>GSMAQILPIRFQEHLQLQNLGINPANIGFSTLTMESDKFICIREKVGEQAQVVIIDMNDPSNPIRRPISADSAIMNPASKVIALKAGKTLQIFNIEMKSKMKAHTMTDDVTFWKWISLNTVALVTDNAVYHWSMEGESQPVKMFDRHSSLAGCQIINYRTDAKQKWLLLTGISAQQNRVVGAMQLYSVDRKVSQPIEGHAASFAQFKMEGNAEESTLFCFAVRGQAGGKLHIIEVGTPPTGNQPFPKKAVDVFFPPEAQNDFPVAMQISEKHDVVFLITKYGYIHLYDLETGTCIYMNRISGETIFVTAPHEATAGIIGVNRKGQVLSVCVEEENIIPYITNVLQNPDLALRMAVRNNLAGAEEL[2x];>ETLLDLDFLE[6x]

Clathrin mediates vesicular transport between post‐Golgi membranes in eukaryotes and is targeted to specific membranes by interactions with clathrin adaptor proteins. A total of 3 consensus clathrin‐binding peptide sequences have been identified and structural studies show that each binds distinct sites on the clathrin heavy chain N‐terminal domain (NTD). We have solved high‐resolution structures of NTD bound to peptide motifs from the cellular clathrin adaptors β2 adaptin and amphiphysin plus a putative viral clathrin adaptor, hepatitis D virus large antigen (HDAg‐L). Surprisingly, with each peptide we observe simultaneous peptide binding at multiple sites on NTD and viral peptides binding to the same sites as cellular peptides.

In addition, to aid comparison with previous biochemical studies, an extended amphiphysin CBM construct (termed Amph4T1) was used in which the clathrin‐binding motif is followed by the amino acids “LERPHRD” arising from the XhoI cloning site and subsequent vector‐derived nucleotides. In all the structures presented a peptide could be observed at the “clathrin box”, lying between blades 1 and 2 of the NTD β‐propeller fold (“clathrin box”). For the cellular peptides (AP2CBMpep, AmphCBMpep and Amph4T1pep) the binding is similar to that previously described, with the 3 leucine side chains of the CBM LΦxΦ[DE] consensus sequence occupying the hydrophobic pocket formed at the groove between the 2 blades. In addition to binding at the clathrin box, we observed significant binding of the cellular peptides (AP2CBMpep, AmphCBMpep and Amph4T1pep) at the “arrestin box”, which lies between blades 4 and 5 of the NTD β‐propeller fold (“arrestin box”). In addition to binding at the clathrin and arrestin boxes, in 3 of the NTD:peptide co‐crystal structures solved (Amph4T1pep, HDAg‐L1pep and HDAg‐L2pep) a bound peptide could be observed lying across the interface between blades 6 and 7 of the NTD β‐propeller. This peptide binding site overlaps with the region identified in the functional studies of Willox and Royle14 as the fourth and final clathrin adaptor binding site on NTD, and we thus henceforth refer to it as the “Royle box” In comparison to surrounding residues, peptides were generally less well‐ordered when bound at this site than when bound at the clathrin box. Binding at the Royle box centres on a deep hydrophobic pocket lying at the interface of blades 6 and 7, formed by the side chains of NTD residues L5, I7, F9, I282, N296 and V327. In the co‐structure with Amph4T1pep a phenylalanine side chain projects deep into this pocket while in the HDAg‐L1pep and HDAg‐L2pep structures the side chains of a leucine residue and proline residue, respectively, bind less deeply.> SSVDDMYDFICSGPLISKIGLTPEKVAESIDEWIEYGLRLCRLFQLNQLSLNEAQKIRIYHYYIPVFMWCEQEISQHSSKFKEEEEIPPLVIGFSAPQGCGKTTLVFALEYLFKITGRKAATMSIDDFYLTAEEQAKLRDSNPGNLLLEFRGNAGSHDLPFSVETMTALSKLTKEGVKVKLPRYDKSAYSGRGDRADPSEWPEVEGPLPVILFEGWMLGFKPLPPEVVKAVDPQLETINKNMEAYYDAWHKYVKSWIVIKIQDPSYVYQWRLQAEIAMRADGKPGMSDEEVKDFV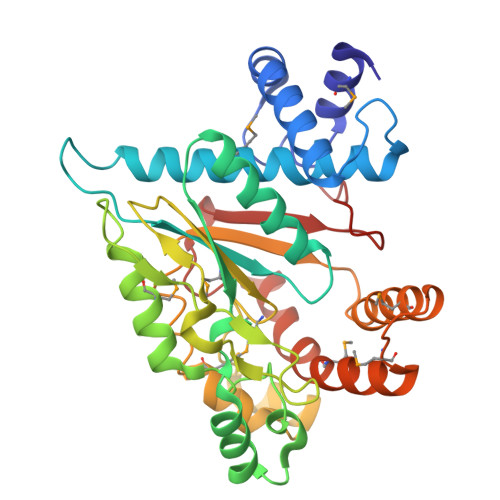SRYMPAYKAYLPTLYSEGPSGSDPKHVLLIDIDEGRNPILGC> GPPMKLRVMEAYPEDVGKGIVRMDKASREKLGVSAGDLVEIKGSKTPMKLRVMEAYPEDVGKGIVRMDKASREKLG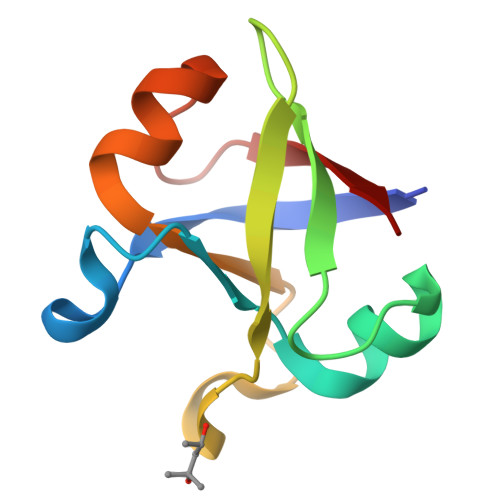VSAGDLVEIKG> GKVA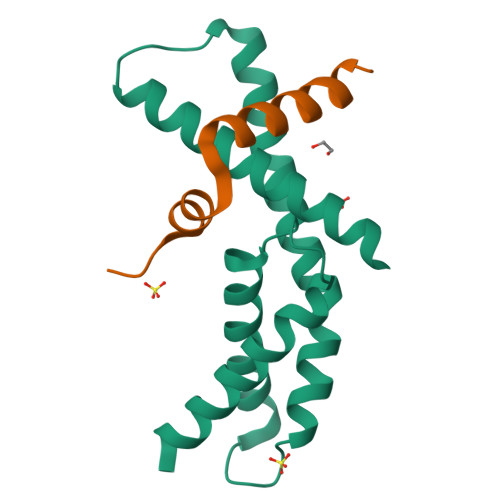LLNAEEEVELAKRIEAGLYATQLMTELSERGEKLPAAQRRDMMWICRDGDRAKNHLLEANLRLVVSLAKRYTGRGMAFLDLIQEGNLGLIRAVEKFDYTKGYKFSTYATWWIRQAITRAMADQAR;> DLAPRQIARYRTDNGEEFEVPFADDAEIPGTWLCRNGMEGTLIEGDLPEPKKVKPPRTHWDMLLERRSIEELEELLKERLELIRSRRRG> VNGAGLLQTVWGPVCELTSELDGQAGAALKKEQEMLAKINDMQMAQLRAAIYL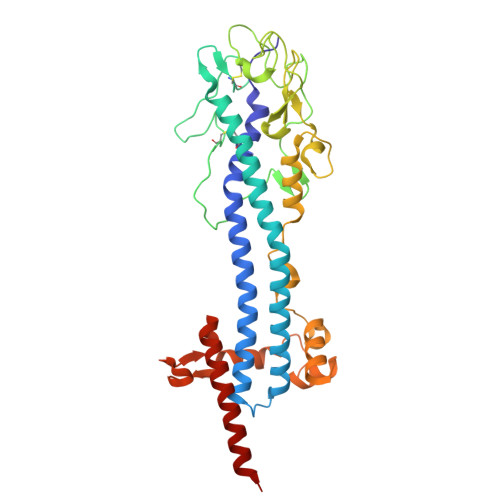AKNPSTPHQNALAVLTAYYAERAGSGKAYFLHALPKAVDSIRRAAYLKGHLDEYLNLLEKSSGGNNKCLVTTDDATVATRGGDQKLAGKNCKLSLSPLKPVDAALTYITKAGVGKLRYDDGGAGGNAVTPSKSGVHACKLLIAHNTAGYGDGGGVTADIDVFAGYMKVKATDAEPKLAAKSDLEEGGGGGAEAWKALHTAIKQEADAEAAELTNETGKLGERRHFLAAATNVLGTGAAGTGNAGRAAVEAAFGSDSEGGDRKIIELIEKELIVKGTANRDADESLGNIKTLKELGELLSYFQLKNSNTINELRNKLKA>MSEQTSSLVIEVMEQQLAKHFQAILQDENRMK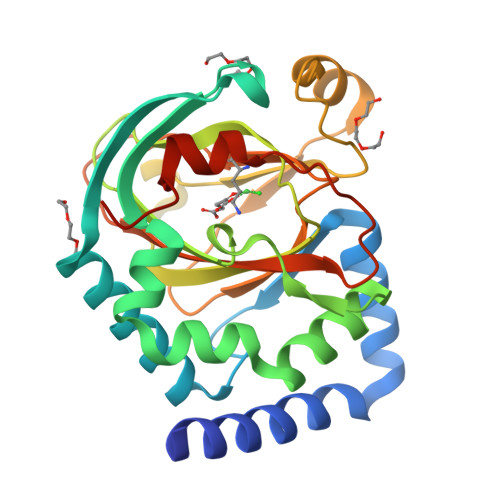QIRNEFRRDGYFNFKNFSFLPKRILENVHAEVHALLDEYSVRRDVTVPSTGNTYRKMYNVNQPEIAEGGTFIPALYQSESLRKFLGNIAGDDLASCWEQEQYLVTKLSHPGDTHGWHWGDYPYTMIWIIEAPEDPAIGGVLQCVPHSEWDKQNPQIWQYILNNPIKSYHHLKGDVYFLKSDTTLHHVVPIQQETTRIILNTCWASAHDRRTDVAHESIEVIWDTKARTTEEA[4x]HYDROXIDE ION | H O | 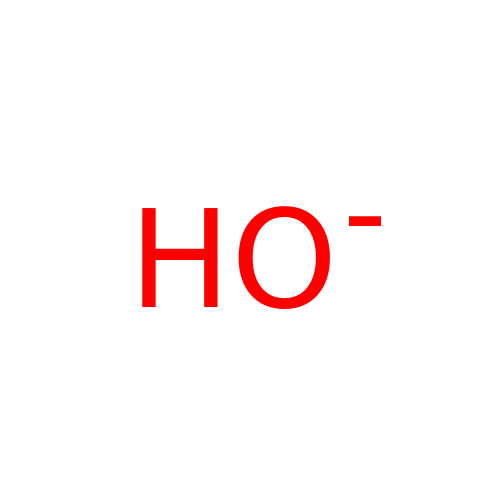XLYOFNOQVPJJNP-UHFFFAOYSA-M However, in the vast majority of prokaryotes, including M. tuberculosis, CoaB and CoaC are encoded by a single gene to produce a fused bifunctional enzyme (CoaBC). CoaBC converts 4′-phosphopantothenate to 4′-phosphopantetheine in three steps. The product of CoaB is then decarboxylated by CoaC, an enzyme of the homo-oligomeric flavin-containing decarboxylase (HFCD) protein family, to 4′-phosphopantetheine. Transcriptional silencing of individual genes of the CoA biosynthetic pathway of this pathogen identified CoaBC as uniquely bactericidal within the CoA pathway, highlighting it as a good candidate for drug discovery.

Screening for crystallisation conditions allowed us to find a different CTP containing condition that gave excellent resolution (1.8 Å). The small differences (RMSD = 1.147 Å) in overall structure of CoaB dimers in the full-length MsmCoaBC and the MsmCoaB crystal structure solved at 1.8 Å can be attributed to artefacts of crystal packing. Hence this crystallisation system could be used to validate CoaB inhibitors binding outside of the CTP site. Nevertheless, a flexible loop (residues 362–377) that covers the 4′-phosphopantothenate site, when this substrate binds to the enzyme, can be seen in our MsmCoaB structure, extending away from the active site. A superposition of our MsmCoaB dimer structure with MsmCoaBC shows the loop extending towards the CoaC active site. This long loop (15–16 amino acids) is present in all CoaBCs and it is possible that it helps channelling the substrate from the CoaB to the CoaC active site. The CoaB active site is enclosed by a loop that extends from the opposing protomer. This loop contains a motif “K-X-K-K”, which is widely conserved in bacteria, with few exceptions, and each lysine either interacts directly with the triphosphate group of CTP or through highly coordinated waters. Also observed is the coordination of a cation by the triphosphate group and D281. While magnesium or manganese are the favoured cations for CoaB activity, calcium is observed in our structures instead, due to the high concentration present in the crystallisation condition.

>MAHHHHHHDMAGVKALVTAGGTREPLDPVRFIGNRSSGKQGYAVARVLAQRGADVTLIAGNTAGLIDPAGVEMVHIGSATQLRDAVSKHAPDANVLVMAAAVADFRPAHVAAAKIKKGASEPSSIDLVRNDDVLAGAVRARADGQLPNMRAIVGFAAETGDANGDVLFHARAKLERKGCDLLVVNAVGENRAFEVDHNDGWLLSADGTESALEHGSKTLMATRIVDSIAAFLKSQDG[4x]> XAGWNAYIDNLMADGTCQDAAIVGYKDSPSVWAAVPGKTFVNITPAEVGILVGKDRSSFFVNGLTLGGQKCSVIRDSLLQDG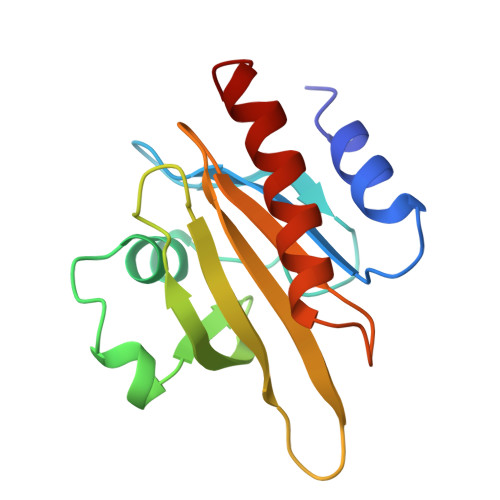EFTMDLRTKSTGGAPTFNITVTMTAKTLVLLMGKEGVHGGMINKKCYEMASHLRRSQY> GSSMDNQDGFILQQVKLSLDDPDSYLSSWNSNDASPCRWSGVSCAGDFSSVTSVDLSSANLAGPFPSVICRLSNLAHLSLYNNSINSTLPLNIAACKSLQTLDLSQNLLTGELPQTLADIPTLVHLDLTGNNFSGDIPASFGKFENLEVLSLVYNLLDGTIPPFLGNISTLKMLNLSYNPFSPSRIPPEFGNLTNLEVMWLTECHLVGQIPDSLGQLSKLVDLDLALNDLVGHIPPSLGGLTNVVQIELYNNSLTGEIPPELGNLKSLRLLDASMNQLTGKIPDELCRVPLESLNLYENNLEGELPASIALSPNLYEIRIFGNRLTGGLPKDLGLNSPLRWLDVSENEFSGDLPADLCAKGELEELLIIHNSFSGVIPESLADCRSLTRIRLAYNRFSGSVPTGFWGLPHVNLLELVNNSFSGEISKSIGGASNLSLLILSNNEFTGSLPEEIGSLDNLNQLSASGNKFSGSLPDSLMSLGELGTLDLHGNQFSGELTSGIKSWKKLNELNLADNEFTGKIPDEIGSLSVLNYLDLSGNMFSGKIPVSLQS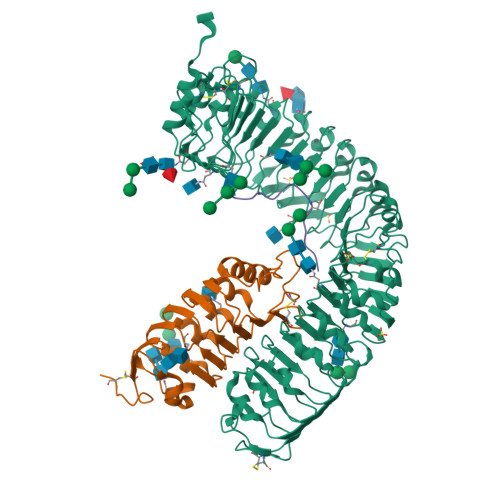LKLNQLNLSYNRLSGDLPPSLAKDMYKNSFIGNPGLCGDIKGLCGSENEAKKRGYVLEGSENLYFQ;> GSSMASANLEGDALHTLRVTLVDPNNVLQSWDPTLVNPCTWFHVTCNNENSVIRVDLGNAELSGHLVPELGVLKNLQYLELYSNNITGPIPSNLGNLTNLVSLDLYLNSFSGPIPESLGKLSKLRFLRLNNNSLTGSIPMSLTNITTLQVLDLSNNRLSGSVPDNGSFSLFTPISFANNLDLCGPVTSHPCPLEGSLENLYFQ;> YVPVPASGPSRKHN>[2x]MTREEARRRINELRDLIRYHNYRYYVLADPEISDAEYDRLLRELKELEERFPEFKSPDSPTEQVGARPLEPTFRPVRHPTRMYSLDNAFTYEEVLAFEERLERALGRKRPFLYTVEHKVDGLSVNLYYEEGVLVFGATRGDGEVGEEVTQNLLTIPTIPRRLKGVPDRLEVRGEVYMPIEAFLRLNEELEERGEKVFKNPRNAAAGSLRQKDPRVTAKRGLRATFYALGLGLEESGLKSQYELLLWLKEKGFPVEHGYEKALGAEGVEEVYRRFLAQRHALPFEADGVVVKLDDLALWRELGYTARAPRFALAYKFPAEEKETRLLDVVFQVGRTGRVTPVGVLEPVFIEGSEVSRVTLHNESYIEELDIRIGDWVLVHKAGGVIPEVLRVLKERRTGEERPIRWPETCPECGHRLVKE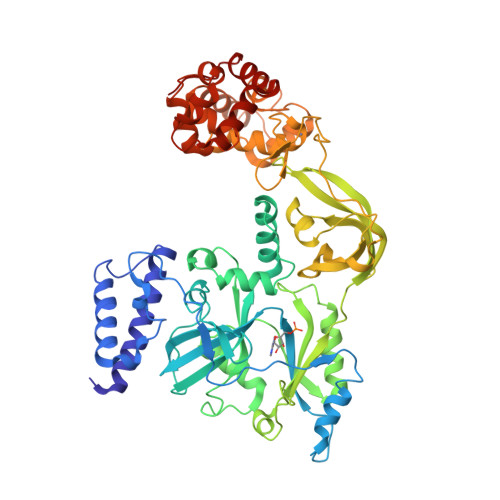GKVHRCPNPLCPAKRFEAIRHYASRKAMDIEGLGEKLIERLLEKGLVRDVADLYHLRKEDLLGLERMGEKSAQNLLRQIEESKHRGLERLLYALGLPGVGEVLARNLARRFGTMDRLLEASLEELLEVEEVGELTARAILETLKDPAFRDLVRRLKEAGVSMESK> MVEQILAEFQLQEEDLKKVMRRMQKEMDRGLRLETHEEASVKMLPTYVRSTPEGSEVGDFLSLDLGGTNFRVMLVKVGEGEEGQWSVKTKHQMYSIPEDAMTGTAEMLFDYISECISDFLDKHQMKHKKLPLGFTFSFPVRHEDIDKGILLNWTKGFKASGAEGNNVVGLLRDAIKRRGDFEMDVVAMVNDTVATMISCYYEDHQCEVGMIVGTGCNACYMEEMQNVELVEG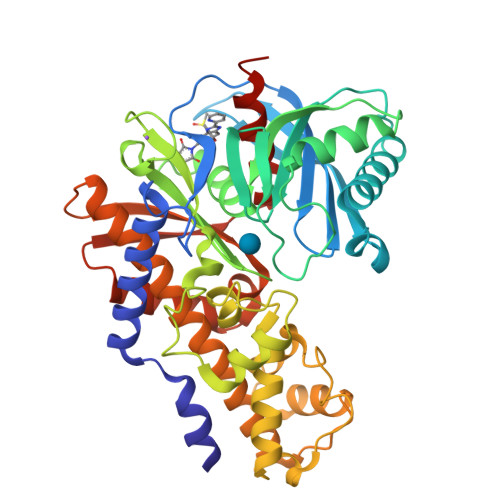DEGRMCVNTEWGAFGDSGELDEFLLEYDRLVDESSANPGQQLYEKLIGGKYMGELVRLVLLRLVDENLLFHGEASEQLRTRGAFETRFVSQVESDTGDRKQIYNILSTLGLRPSTTDCDIVRRACESVSTRAAHMCSAGLAGVINRMRESRSEDVMRITVGVDGSVYKLHPSFKERFHASVRRLTPSCEITFIESEEGSGRGAALVSAVACKKACMLGQ>[2x]M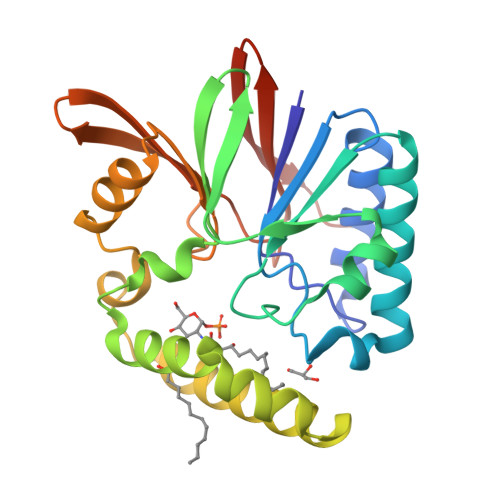SVLFISDLHLEAERPDITRAFLSFLDERARRAEALYILGDFFEAWIGDDGMDAFQRSIAQSLRQVADGGTRIYLMHGNRDFLIGKAFCREAGCTLLPDPSVIDLYGEPVLLMHGDSLCTRDEAYMRLRRWLRNPLTLWVLRHLPLATRHKLARKLRKESRAQTRMKAVDIIDVTPEEVPRVMRGHGVRTLIHGHTHRPAEHPLDIDGQPARRIVLGDWDRQGWALEIDANGHRQAPFPLLEHHHHHH GSTs are a multifunctional superfamily of enzymes, distributed in all major kingdoms of living organisms. They are long established to catalyze the conjugation of the tripeptide glutathione with diverse electrophilic and hydrophobic compounds, resulting in their modification to display higher solubility and less toxicity. GSTs that belong to the phi class are dimeric enzymes, comprised of two identical subunits. Residues of the N-terminal domain residues assist the formation of a GSH binding site (G-site), whereas hydrophobic residues of the C-terminal domain form the hydrophobic substrate binding site (H-site).

The structures of sh101 and sh155 enzyme variants were resolved at 1.87 and 2.00 Å resolution and compared to the wild-type AmGSTF enzyme structure that has been recently reported. Sh101 and sh155 were crystallized with two and three molecules in the asymmetric unit, respectively. The sequence between the β2 and β3 strands where the α2 helix is located exhibits significant distortion due to high flexibility. This part has not been modelled in sh101 because of the high flexibility and lack of electron density. Amino acid sequence alignments of the sh101 with the parent enzyme AmGSTF showed 94.98% identity. For instance, the region Tyr118-Arg127 has three substitutions in sh101 sequence (Gln119Glu, Phe122Ile, Met125Leu), as a result of the replacement of the C-terminal part of the α4 helix by the sequence derived from the crop-type GSTFs (TdGSTF and HvGSTF). Among the selected enzymes, sh101 and sh155 exhibited the highest improvement in kcat values (185.9 ± 1.8 min−1 and 197.7 ± 3.2 min−1, respectively), corresponding to an approximately 5-fold improvement, compared to the wild-type AmGSTF enzyme (35.9 ± 1.7 min−1). Furthermore, the sh101 enzyme exhibited lower S0.5 and Km values towards CDNB, leading to significant improvement (7–8 times) in catalytic efficiency compared to the parent enzyme AmGSTF. In particular, the Tm values of sh101 and sh155 enzyme variants were significantly increased by 8.3 and 5.2 °C compared to the parent enzyme AmGSTF. Inspection of the crystal structures of sh101 and sh155 shows that Lys93 can form a new salt bridge with Asp62 of the opposite subunit.

>[2x]MAPVKVFGPAMSTNVARVTLCLEEVGAEYEVVNIDFNTMEHKSPEHLARNPFGQIPAFQDGDLLLWESRAISKYVLRKYKTDEVDLLREGNLKEAAMVDVWTEVDAHTYNPALSPIVYECLINPLMRGLPTNQTVVDESLEKLKKVLEVYEARLSQHKYLAGDFVSFADLNHFPYTFYFMATPHAALFDSYPHVKAWWDRLMARPAVKKIAATMVPPKAHHHHHH> MSLSNCLHKPDEERTKEKHVPEMKLSGNHVDIRCGATVMHPATEKHYIGTIRLFGITKEGNV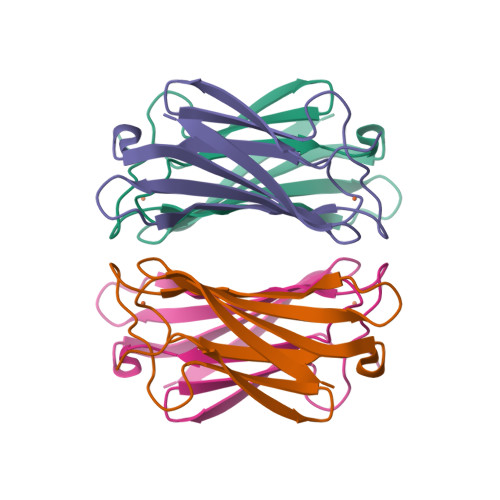TLELGCQQIWPGLGEPVASFRVCDLEKYKGLLAVAYCNLHGCWENYMEL> MNFGAFSINPAMMAAAQAALQSSWGMMGMLASQQNQSGPSGNN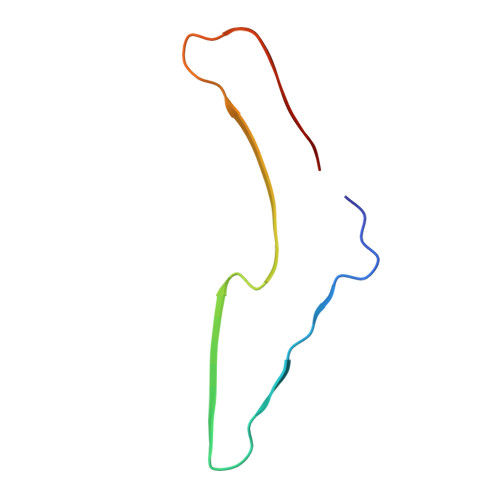QNQGNMQ> TPTTFVHLFEWNWQDVAQECEQYLGPKGYAAVQVSPPNEHITGSQWWTRYQPVSYELQSRGGNRAQFIDMVNRCSAAGVDIYVDTLINHMAAGSGTGTAGNSFGNKSFPIYSPQDFHESCTINNSDYGNDRYRVQNCELVGLADLDTASNYVQNTIAAYINDLQAIGVKGFRFDASKHVAASD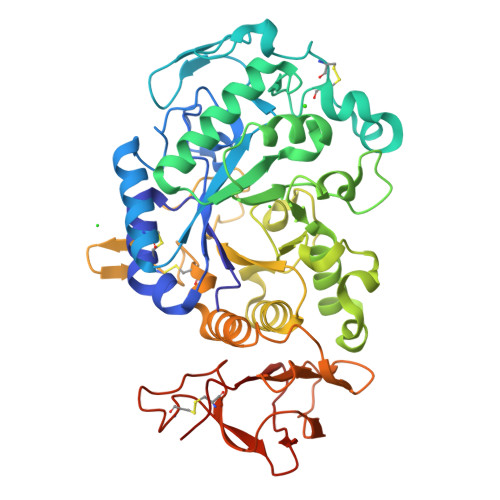IQSLMAKVNGSPVVFQEVIDQGGEAVGASEYLSTGLVTEFKYSTELGNTFRNGSLAWLSNFGEGWGFMPSSSAVVFVDNHDNQRGHGGAGNVITFEDGRLYDLANVFMLAYPYGYPRVMSSYDFHGDTDAGGPNVPVHNNGNLECFASNWKCEHRWSYIAGGVDFRNNTADNWAVTNWWDNTNNQISFGRGSSGHMAINKEDSTLTATVQTDMASGQYCNVLKGELSADAKSCSGEVITVNSDGTINLNIGAWDAMAIHKNAKLNTSSAS> 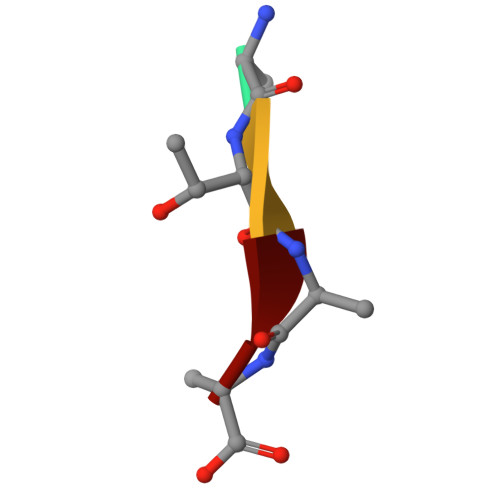ATAA>TYFITMNNARNFFIQQLESNAQDTATSLGLSLSQSLINHDVPTMDSMVKAVFDRGYFSSIKVQDIKGKVIILKKQLPQESDIPQWFVNLIKWPSTEKSSLIMDGWMQAGVVLVASDPSYVYASLWRNAVEM[4x];>ADWDFSAISRKATALYGPLGAGQQRIDAWQNLLATQKQVSEMEKLKVVNLFFNKQMRYVEDIDLWHEVDYWETPIEALWKGAGDCEDYAIAKYFSLRHLGVASDKLRITYVKALRQNRAHMVLTYYSSPDAMPLVLDSLIDPIKPAAERTDL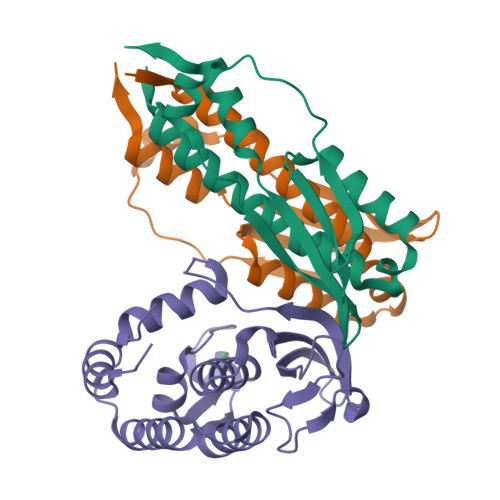LPVYSFNAEGLYLPGAKGNKKVGDTKRLSRWQDVLKKMQAEGFPV[2x]> AMDPPHRPRPGAFRGGERVVHPRFGPGTVVAAQGDEVTVHFEGFGLKRLSLKYAELK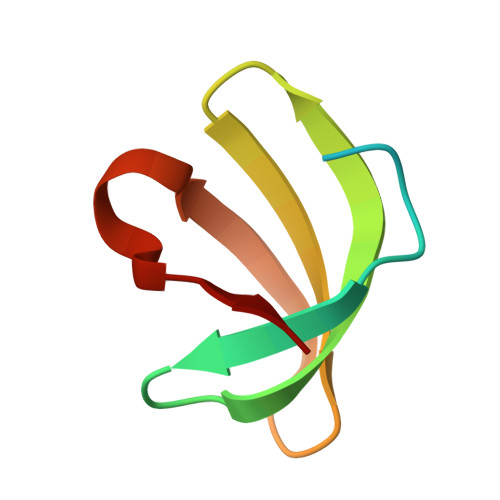PA> ATALAEMPKRKFTIDDFDIGRPLGKGKFGNVYLAREKQNKFIMALKVLFKSQLEKEGVEHQLRREIEIQSHLRHPNILRMYNYFHDRKRIYLMLEFAPRGELYKELQKHGRFDEQRSATFMEELADALHYCHERKVIHRDIKPENLLM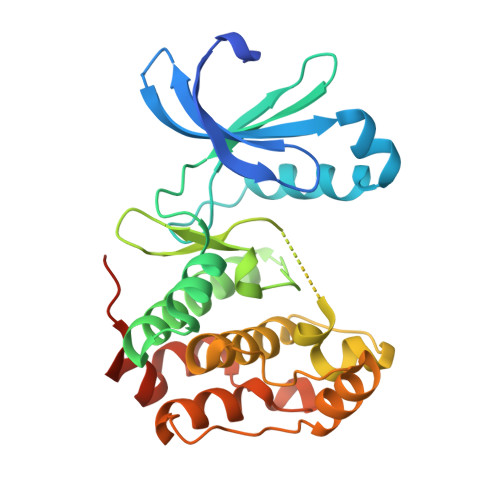GYKGELKIADFGWSVHAPSLRRRTMCGTLDYLPPEMIEGKTHDEKVDLWCAGVLCYEFLVGMPPFDSPSHTETHRRIVNVDLKFPPFLSDGSKDLISKLLRYHPPQRLPLKGVMEHPWVKANSRRVLPGVYQSTQSKD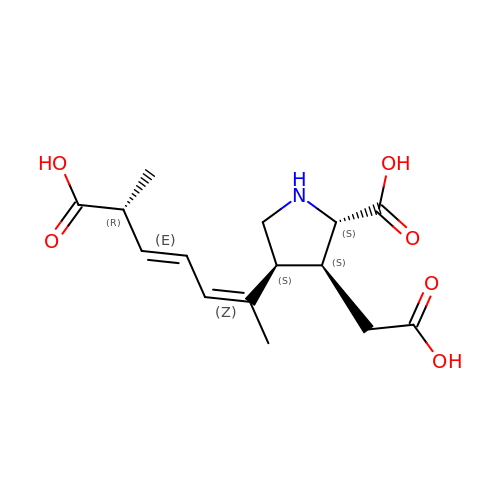(2S,3S,4S)-2-CARBOXY-4-[(1Z,3E,5R)-5-CARBOXY-1-METHYL-1,3-HEXADIENYL]-3-PYRROLIDINEACETIC ACID | C15 H21 N O6 | VZFRNCSOCOPNDB-AOKDLOFSSA-N> GPGSMAASRRLMKELEEIRKCGMKNFRNIQVDEANLLTWQGLIVPDNPPYDKGAFRIEINFPAEYPFKPPKITFKTKIYHPNIDEKGQVCLPVISAENWKPATKTDQVIQSLIALVNDPQPEHPLRADLAEEYSKDRKKFCKNAEEFTKKYGEKRPVD;> GPGSEFQECAVCG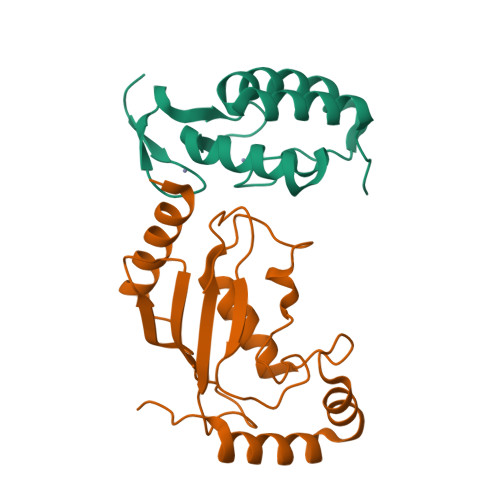WALPHNRMQALTSCECTICPDCFRQHFTIALKEKHITDMVCPACGRPDLTDDTQLLSYFSTLDIQLRESLEPDAYALFHKKLTEGVLMRD N-[1H-INDOL-3-YL-ACETYL]GLYCINE ACID | C12 H12 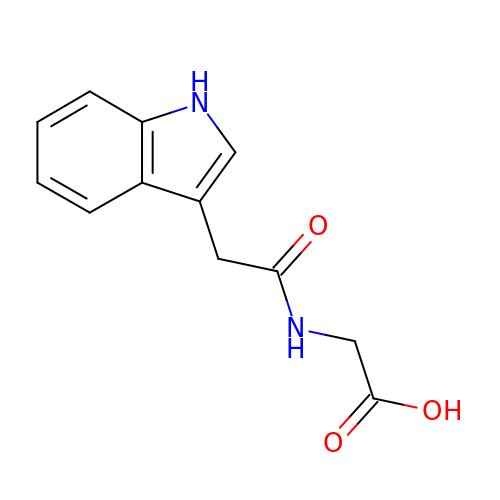N2 O3 | YDXXLJMIHMIOIF-UHFFFAOYSA-N>MKTINSVDTKEFLNHQVANLNVFTVKIHQIHWYMRGHNFFTLHEKMDDLYSEFGE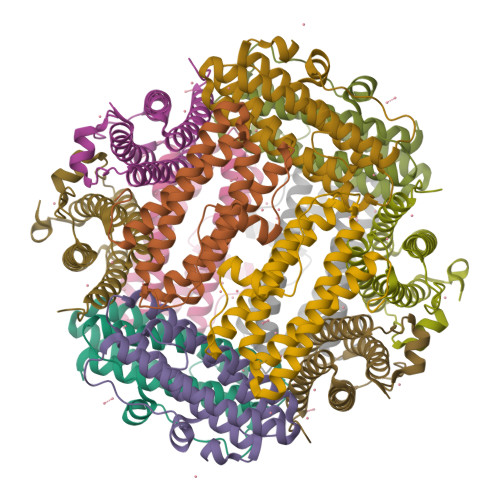QMDEVAERLLAIGGSPFSTLKEFLENASVEEAPYTKPKTMDQLMEDLVGTLELLRDEYKQGIELTDKEGDDVTNDMLIAFKASIDKHIWMFKAFLGKAPLE[6x]>SNAMSELSYRRILLKLSGEALMGDGDYGIDPKVINRLAHEVIEAQQAGAQVALVIGGGNIFRGAGLAASGMDRVTGDHMGMLATVINALAMQDALEKLGAKVRVMSAIKINDVCEDFIRRRAIRHLEKGRIAIFAAGTGNPFFTTDSGAALRAIEIGADLLLKATKVDGVYDKDPKKHSDAVRYDSLTYDEVIMQGLEVMDTAAFALARDSD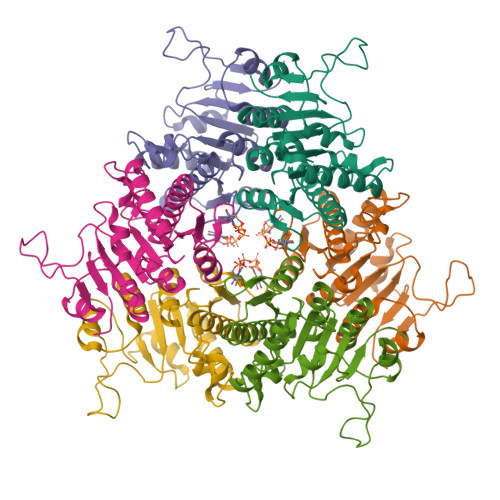LPLRIFGMSEPGVLLRILHGAQIGTLVQGRS[6x]>MLVWLAEHLVKYYSGFNVFSYLTFRAIVSLLTALFISLWMGPRMIAHLQKLSFGQVVRNDGPESHFSKRGTPTMGGIMILTAIVISVLLWAYPSNPYVWCVLVVLVGYGVIGFVDDYRKVVRKDTKGLIARWKYFWMSVIALGVAFALYLAGKDTPATQLVVPFFKDVMPQLGLFYILLAYFVIVGTGNAVNLTDGLDGLAIMPTVFVAGGFALVAWATGNMNFASYLHIPYLRHAGELVIVCTAIVGAGLGFLWFNTYPAQVFMGDVGSLALGGALGIIAVLLRQEFLLVIMGGVFVVETLSVILQVGSFKLRGQRIFRMAPIHHHYELKGWPEPRVIVRFWIISLMLVLIGLATLKVR[2x];>[2x]MGVRWTLWDTLAFLLLLSLLLPSLLIMFIPSTFKRPVSSWKARNLRKTLLMASSVRLKPLNCSRLPCVYAQETLTFLLTQKKTCVKNYVRKEHHHHHH;>[2x]MKVAKDLVVSLAYQVRTEDGVLVDESPVSAPLDYLHGHGSLISGLETALEGHEVGDKFDVAVGANDAYGQYDENLVQRVPKDVFMGVDELQVGMRFLAETDQGPVPVEITAVEDDHVVVDGNHMLAGQNLKFNVEVVAIREATEEELAH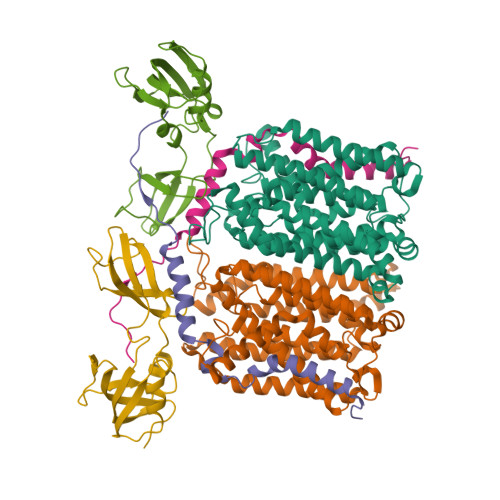GHVHG> APNDQHYREQWHYFDRYGVKADKVWDMGFTGQNVVVAVVDTGILHHRDLNANVLPGYDFISNSQISLDGDGRDADPFDEGDWFDNWACGGYPDPRKERSDSSWHGSHVAGTIAAVTNNRIGVAGVAYGAKVVPVRALGRCGGYDSDISDGLYWAAGGRIAGI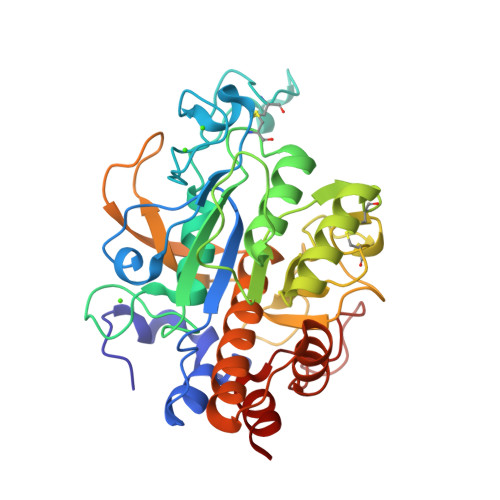PENRNPAKVINMSLGSDGQCSYNAQTMIDRATRLGALVVVAAGNENQNASNTWPTSCNNVLSVGATTSRGIRASFSNYGVDVDLAAPGQDILSTVDSGTRRPVSDAYSFMAGTSMATPHVSGVAALVISAANSVNKNLTPAELKDVLVSTTSPFNGRLDRALGSGIVDAEAAVNSVLG>DDNGIVLLGERAAKCRAYAKALHYKELEFQKGPTPAILESLISINNKLQQPEAAAGVLEYAMKHFGELEIQATWYEKLHEWEDALVAYDKKMDTNKDDPELMLGRMRCLEALGEWGQLHQQCCEKWTLVNDETQAKMARMAAAAAWGLGQWDSMEEYTCMIPRDTHDGAFYRAVLALHQDLFSLAQQCIDKARDLLDAELTAMAGESYSRAYGAMVSCHMLSELEEVIQYKLVPERREIIRQIWWERLQGCQRIVEDWQKILMVRSLVVSPHEDMRTWLKYASLCGKSGRLALAHKTLVLLLGVDPSRQLDHPLPTVHPQVTYAYMKNMWKSARKIDAFQHMQHFVQTMQQQAQHAIATEDQQHKQELHKLMARCFLKLGEWQLNLQGINESTIPKVLQYYSAATEHDRSWYKAWHAWAVMNFEAVLHYKHQNQARDEKKKLRHASGANITNATTAATTAATATTTASTEGSNSESEAESTENSPTPSPLQKKVTEDLSKTLLMYTVPAVQGFFRSISLSRGNNLQDTLRVLTLWFDYGHWPDVNEALVEGVKAIQIDTWLQVIPQLIARIDTPRPLVGRLIHQLLTDIGRYHPQALIYPLTVASKSTTTARHNAANKILKNMCEHSNTLVQQAMMVSEELIRVAILWHEMWHEGLEEASRLYFGERNVKGMFEVLEPLHAMMERGPQTLKETSFNQAYGRDLMEAQEWCRKYMKSGNVKDLTQAWDLYYHVFRRISKQLPQLTSLELQYVSPKLLMCRDLELAVPGTYDPNQPIIRIQSIAPSLQVITSKQRPRKLTLMGSNGHEFVFLLKGHEDLRQDERVMQLFGLVNTLLANDPTSLRKNLSIQRYAVIPLSTNSGLIGWVPHCDTLHALIRDYREKKKILLNIEHRIMLRMAPDYDHLTLMQKVEVFEHAVNNTAGDDLAKLLWLKSPSSEVWFDRRTNYTRSLAVMSMVGYILGLGDRHPSNLMLDRLSGKILHIDFGDCFEVAMTREKFPEKIPFRLTRMLTNAMEVTGLDGNYRITCHTVMEVLREHKDSVMAVLEAFVYDPLLNWRLMDTNTKGNKRSRTRTDSYSAGQSVEILDGVELGEPAHKKTGTTVPESIHSFIGDGLVKPEALNKKAIQIINRVRDKLTGRDFSHDDTLDVPTQVELLIKQATSHENLCQCYIGWCPFW[2x];>MNTSPGTVGSDPVILATAGYDHTVRFWQAHSGICTRTVQHQDSQVNALEVTPDRSMIAAAGYQHIRMYDLNSNNPNPIISYDGVNKNIASVGFHEDG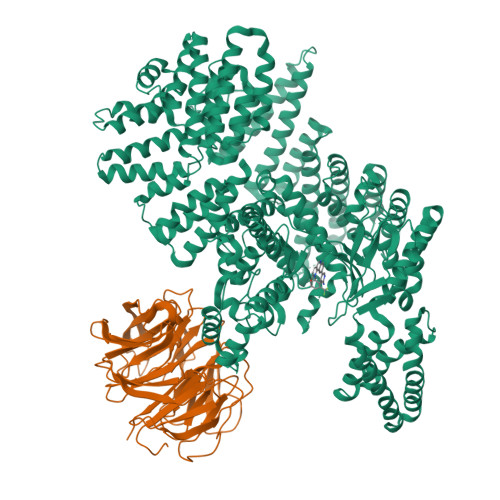RWMYTGGEDCTARIWDLRSRNLQCQRIFQVNAPINCVCLHPNQAELIVGDQSGAIHIWDLKTDHNEQLIPEPEVSITSAHIDPDASYMAAVNSTGNCYVWNLTGGIGDEVTQLIPKTKIPAHTRYALQCRFSPDSTLLATCSADQTCKIWRTSNFSLMTELSIKSGNPGESSRGWMWGCAFSGDSQYIVTASSDNLARLWCVETGEIKREYGGHQKAVVCLAFNDSVLG[2x]Interleukin-1 receptor associated kinases (IRAKs) are key players in innate immune signaling that mediate the host response to pathogens. In contrast to the active kinases IRAK1 and IRAK4, IRAK2 and IRAK3 are pseudokinases lacking catalytic activity and their functions are poorly understood. IRAK3 is thought to be a negative regulator of innate immune signaling and mutations in IRAK3 are associated with asthma and cancer. The canonical catalytic “HRD”-motif is missing entirely in IRAK3 and replaced with “CGS,” whereas the Mg2+-coordinating “DFG”-motif is slightly altered to “DFA.

Here we report the crystal structure of the pseudokinase domain of human IRAK3 at 2.9 Å resolution, which reveals a closed, pseudoactive conformation with an evolutionarily conserved cysteine residue located in the regulatory spine (R-spine). The asymmetric unit (ASU) contains 3 molecules of IRAK3. The αC-helix of IRAK3 is in an inward-oriented position with an intact KE-salt bridge formed by K192 of the β3-strand and E212 of the αC-helix. Another hallmark of an active kinase conformation in IRAK3 is the intact regulatory spine (R-spine) formed by L227, L216, F312, C291, and L309. The presence of this evolutionarily conserved cysteine residue in the R-spine of IRAK3 suggests the possibility of a redox-based mechanism that controls R-spine assembly. Closer inspection of the G-loop interactions in the IRAK3 structure revealed that F177 anchors the G-loop to residues of the αC-helix, β3-and β4-strands and to the Mg-binding loop. The hydrophobic anchor F177 thereby leads to a rigidification of the G-loop and keeps the loop ordered in the apo-form of IRAK3. The dimers are formed via a pseudosymmetric “head-to-head” arrangement with the αC-helices as central elements of the dimer interface. The interface is flanked by two disulfide bonds formed between C202 at the start of the αC-helices and C287 of the αE-β6-loops. We further identify a conserved C-lobe surface on IRAK3 that harbors asthma-associated mutations and closely resembles the previously reported IRAK4 homodimer interface.

>[3x]GPLGSKGVLLKSSISFQNIIEGTRNFHKDFLIGEGEIFEVYRVEIQNLTYAVKLFKQEKKMQCKKHWKRFLSELEVLLLFHHPNILELAAYFTETEKFCLIYPYMRNGTLFDRLQCVGDTAPLPWHIRIGILIGISKAIHYLHNVQPCSVICGSISSANILLDDQFQPKLTDFAMAHFRSHLEHQSCTINMTSSSSKHLWYMPEEYIRQGKLSIKTDVYSFGIVIMEVLTGCRVVLDDPKHIQLRDLLRELMEKRGLDSCLSFLDKKVPPCPRNFSAKLFCLAGRCAATRAKLRPSMDEVLNTLESTQASLYFAE> HGEKSQQAFLRMRTLNWYDVQWSKTT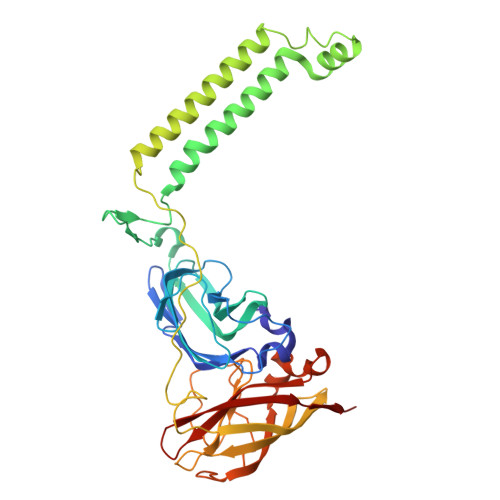VNVNEEMVLSGKVHVFSAWPQAVANPRVSFLNAGEPGPVLVRTAQFIGEQFAPRSVSLEIGKDYAFSINLRGRRAGRWHVHAQINVEGGGPIIGPGQWIEIKGDMKDFTDPVTLLDGSTVDLEHYGISRVYAWHLPWMAVGAAWIFFWFVRKGIITSYIRVAEGKADDVIGDDDRRIGAIVLALTILATIVGYAVTNSTFPRTIPLQAGLQKPLTPIETEGTVGVGKENVTTELNGGVYKVPGRELTINVKVKNNTSQPLRLGEYTAAGLRFLNPDVFTTKPDFPDYLLADRGLSVDATPIAPGEAKEIVVKIQDARWDIERLSDLAYDTDSQIGGLLFFFSPDGKRYASEIGGPVIPKFVA> NVIQDLYLRELKDTKLAPSTLQDAEGNVKPWNPPQKPNLPELELQGPEALKAYTEQNVETAHVAKESEEGESEPIEEDWLVLDDAEETKESH;> SLAKSAANKLDWAKVISSLRITGSTATQLSSFKKRNDEARRQLLELQSQPTEVDFSHYRSVLKNTSVIDKIESYVKQYKPVKIDASKQLQVIESFEKHAMTNAKETESLVSKELKDLQSTLDNIQSARPFDELTVDDLTKIKPEIDAKVEEMVKKGKWDVPGYKDRFGNLNVM;> MPQLVPFYFMNQLTYGFLLMITLLILFSQFFLPMILRLYVSRLFISKL;>[3x]ASTKAQPTEVSSILEERIKGVSDEANLNETGRVLAVGDGIARVFGLNNIQAEELVEFSSGVKGMALNLEPGQVGIVLFGSDRLVKEGELVKRTGNIVDVPVGPGLLGRVVDALGNPIDGKGPIDAAGRSRAQVKAPGILPRRSVHEPVQTGLKAVDALVPIGRGQRELIIGDRQTGKTAVALDTILNQKRWNNGSDESKKLYCVYVA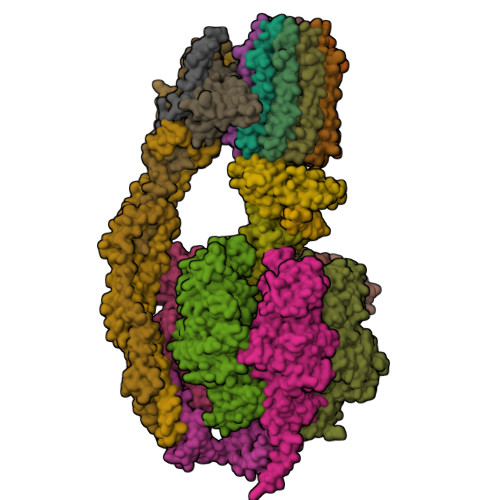VGQKRSTVAQLVQTLEQHDAMKYSIIVAATASEAAPLQYLAPFTAASIGEWFRDNGKHALIVYDDLSKQAVAYRQLSLLLRRPPGREAYPGDVFYLHSRLLERAAKLSEKEGSGSLTALPVIETQGGDVSAYIPTNVISITDGQIFLEAELFYKGIRPAINVGLSVSRVGSAAQVKALKQVAGSLKLFLAQYREVAAFAQFGSDLDASTKQTLVRGERLTQLLKQNQYSPLATEEQVPLIYAGVNGHLDGIELSRIGEFESSFLSYLKSNHNELLTEIREKGELSKELLASLKSATESFVATF;>[3x]ASAAQSTPITGKVTAVIGAIVDVHFEQSELPAILNALEIKTPQGKLVLEVAQHLGENTVRTIAMDGTEGLVRGEKVLDTGGPISVPVGRETLGRIINVIGEPIDERGPIKSKLRKPIHADPPSFAEQSTSAEILETGIKVVDLLAPYARGGKIGLFGGAGVGKTVFIQELINNIAKAHGGFSVFTGVGERTREGNDLYREMKETGVINLEGESKVALVFGQMNEPPGARARVALTGLTIAEYFRDEEGQDVLLFIDNIFRFTQAGSEVSALLGRIPSAVGYQPTLATDMGLLQERITTTKKGSVTSVQAVYVPADDLTDPAPATTFAHLDATTVLSRGISELGIYPAVDPLDSKSRLLDAAVVGQEHYDVASKVQETLQTYKSLQDIIAILGMDELSEQDKLTVERARKIQRFLSQPFAVAEVFTGIPGKLVRLKDTVASFKAVLEGKYDNIPEHAFYMVGGIEDVVAKAEKLAAEAN;> ATLKEVEMRLKSIKNIEKITKTMKIVASTRLSKAEKAKISAKKMDEAEQLFYKNAETKNLDVEATETGAPKELIVAITSDKGLCGSIHSQLAKAVRRHLNDQPNADIVTIGDKIKMQLLRTHPNNIKLSINGIGKDAPTFQESALIADKLLSVMKAGTYPKISIFYNDPVSSLSFEPSEKPIFNAKTIEQSPSFGKFEIDTDANVPRDLFEYTLANQMLTAMAQGYAAEISARRNAMDNASKNAGDMINRYSILYNRTRQAVITNELVDIITGASSLG;> AEAAAASSGLKLQFALPHETLYSGSEVTQVNLPAKSGRIGVLANHVPTVEQLLPGVVEVMEGSNSKKFFISGGFATVQPDSQLCVTAIEAFPLESFSQENIKNLLAEAKKNVSSSDAREAAEAAIQVEVLENLQSVLK;> SAWRKAGISYAAYLNVAAQAIRSSLKTELQTASVLNRSQTDAFYTQYKNGTAASEPTPITK;> MLKRFPTPILKVYWPFFVAGAAVYYGMSKAADLSSNT;>MQLVLAAKYIGAGISTIGLLGAGIGIAIVFAALINGVSRNPSIKDTVFPMAILGFALSEATGLFCLMVSFLLLFGV[10x];> VSTLIPPKVVSSKNIGSAPNAKRIANVVHFYKSLPQGPAPAIKANTRLARYKAKYFDGDNASGKPLWHFALGIIAFGYSMEYYFHLRHHKGAEEH;> SPLDQFEIRTLFGLQSSFIDLSCLNLTTFSLYTIIVLLVITSLYTLTNNNNKIIGSRWLISQEAIYDTIMNMTKGQIGGKNWGLYFPMIFTLFMFIFIANLISMIPYSFALSAHLVFIISLSIVIWLGNTILGLYKHGWVFFSLFVPAGTPLPLVPLLVIIETLSYFARAISLGLRLGSNILAGHLLMVILAGLTFNFMLINLFTLVFGFVPLAMILAIMMLEFAIGIIQGYVWAILTASYLKDAVYLH;> ASKAAAPPPVRLFGVEGTYATALYQAAAKNSSIDAAFQSLQKVESTVKKNPKLGHLLLNPALSLKDRNSVIDAIVETHKNLDGYVVNLLKVLSENNRLGCFEKIASDFGVLNDAHNGLLKGTVTSAEPLDPKSFKRIEKALSASKLVGQGKSLKLENVVKPEIKGGLIVELGDKTVDLSISTKIQKLNKVLEDSI;> MSSTPEKQTDPKAKANSIINAIPGNNILTKTGVLGTSAAAVIYAISNELYVINDESILLLTFLGFTGLVAKYLAPAYKDFADARMKKVSDVLNASRNKHVEAVKDRIDSVSQLQNVAETTKVLFDVSKETVELESEAFELKQKVELAHEAKAVLDSWVRYEASLRQLEQRQLAKSVISRVQSELGNPKFQEKVLQQSISEIEQLLSKLK>[2x]SMNKKTKLIHGGHTTDDYTGAVTT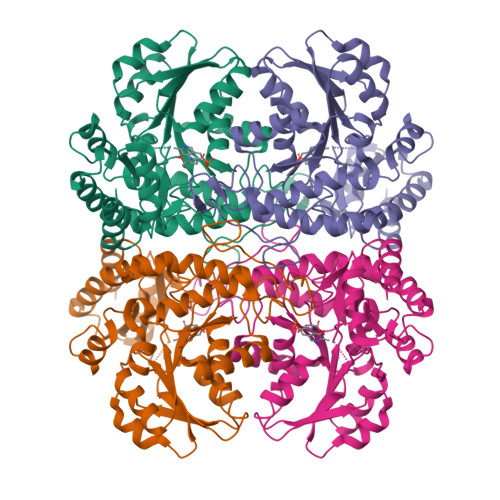PIYQTSTYLQDDIGDLRQGYEYSRTANPTRSSVESVIAALENGKHGFAFSSGVAAISAVVMLLDKGDHIILNSDVYGGTYRALTKVFTRFGIEVDFVDTTHTDSIVQAIRPTTKMLFIETPSNPLLRVTDIKKSAEIAKEHGLISVVDNTFMTPYYQNPLDLGIDIVLHSATAYLGGHSDVVAGLVATSDDKLAERLAFISNSTGGILGPQDSYLLVRGIKTLGLRMEQINRSVIEIIKMLQAHPAVQQVFHPSIESHLNHDVHMAQADGHTGVIAFEVKNTESAKQLIKATSYYTLAESLGAVESLISVPALMTHASIPADIRAKEGITDGLVRISVGIEDTEDLVDDLKQALDTL> ESQPD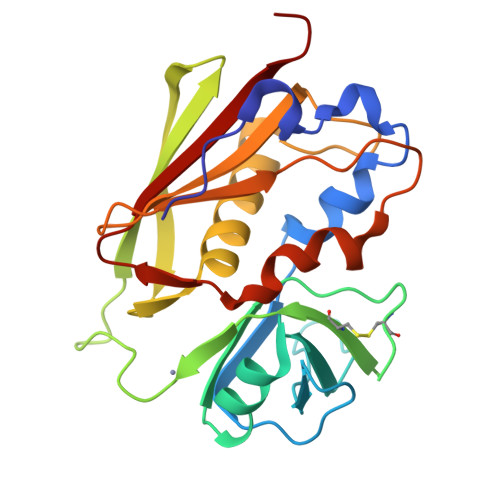PMPDDLHKSSEFTGTMGNMKYLYDDHYVSATKVKSVDKFLAHDLIYNISDKKLKNYDKVKTELLNEDLAKKYKDEVVDVYGSNYYVNCYFSSKDASTWHGKTCMYGGITKHEGNHFDNGNLQNVLVRVYENKRNTISFEVQTDKKSVTAQELDIKARNFLINKKNLYEFNSSPYETGYIKFIENNGNTFWYDMMPAPGDKFDQSKYLMMYNDNKTVDSKSVKIEVHLTTKNG>[12x]MEKFLVIAGPNAIESEELLLKVGEEIKRLSEKFKEVEFVFKSSFDKANRSSIHSFRGHGLEYGVKALRKVKEEFGLKITTDIHESWQAEPVAEVADIIQIPAFLCRQTDLLLAAAKTGRAVNVKKGQFLAPWDTKNVVEKLKFGGAKEIYLTERGTTFGYNNLVVDFRS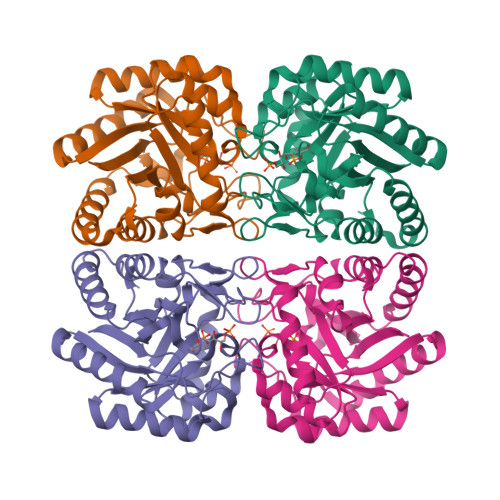LPIMKQWAKVIYDATHSVQLPGGLGDKSGGMREFIFPLIRAAVAVGCDGVFMETHPEPEKALSDAPTALPLSQLEGIIEAILEIREVASKYYETIPVK1-({2-[2-(4-CHLOROPHENYL)ETHYL]-1,3-DIOXOLAN-2-YL}METHYL)-1H-IMIDAZOLE | C15 H17 Cl N2 O2 | 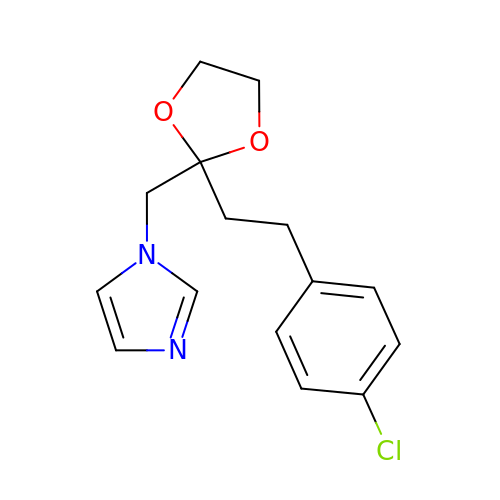NPIOYRIZNLPLDH-UHFFFAOYSA-N>[4x]MAHHHHHHMPVIRDFQPADIETITAIYTQAVLTGTGSYEIEPPTMDEMAKRFAAFADQGFPILVAEADG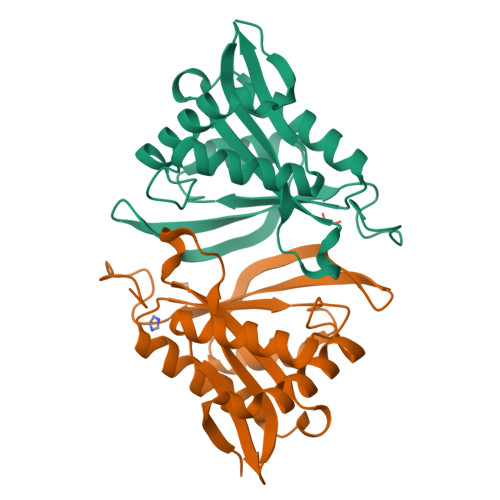RVLGYAYASYFRVRPAYRWLAEDSIYIAPDAKGQGIGKLLLRELIARISALGFRQLLAVIGDGEHNIGSVKLHESLGFTHCGRIEGSGFKHGRWLDTVLMQLPLNGGRSTEPGPSPLS> NSCTHFPGNLPNMLRDLRDAFSRVKTFFQMKDQLDNLLLKESLLEDFKGYLGCQALSEMIQFYLEEVMPQAENQDPDIKAHVNSLGENLKTLRLRLRRCHRFLPCENKSKAVEQVKNAFNKLQEKGIYKAMSEFDIFINYIEAY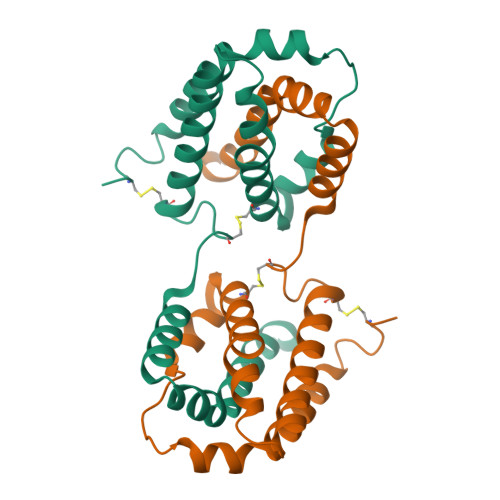MTMKIRN>[3x]ATDGSHFDFVIVGGGTAGNTVAGR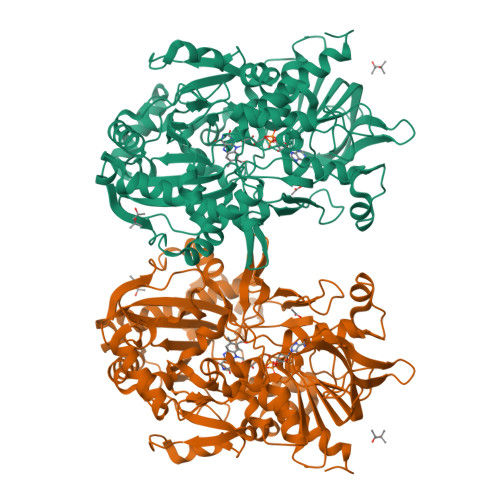LAENPNVTVLIVEAGIGNPEDIPEITTPSSAMDLRNSKYDWAYKTTMVRRDDYERIEKPNTRGKTLGGSSSLNYFTWVPGHKATFDQWEEFGGKEWTWDPLVPYLRKSATYHDDPRLYSPELEKIGGGGPIPISHAELIDEMAPFRENLTKAWKSMGQPLIENIYDGEMDGLTHCCDTIYRGQRSGSFLFVKNKPNITIVPEVHSKRLIINEADRTCKGVTVVTAAGNELNFFADREVILSQGVFETPKLLMLSGIGPTRELSRHGINTIVDSRHVGQNLMDHPGVPFVLRVKDGFGMDDVLLRHGPKRDAVVSAYNKNRSGPVGSGLLELVGFPRIDKYLEKDAEYRKAKAANGGKDPFSPLGQPHFELDFVCMFGTAFQWHFPTPKTGDHLTVVVDLVRPISDPGEVTLNSADPFQQPNINLNFFANDLDIIAMREGIRFSYDLLFKGEGFKDLVESEYPWEMPLDSDKEMHRAVLDRCQTAFHPTGTARLSKNIDQGVVDPKLKVHGIKKLRVADASVIPIIPDCRIQNSVYAVGEKCADMIKAEHKDLY>ETPVLEKNNVTLTGGGENVTKELKDKFTSGDFTVVIKYNQSSEKGLQALFGISNSKPGQQNSYVDVFLRDNGELGMEARDTSSNKNNLVSRPASVWGKYKQEAVTNTVAVVADSVKKTYSLYANGTKVVEKKVDNFLNIKDIKGIDYYMLGGVKRAGKTAFGFNGTLENIKFFNSALDEETVKKMTTNAVTGHLIYTANDTTGSNYFRIPVLYTFSNGRVFSSIDARYGGTHDFLNKINIATSYSDDNGKTWTKPKLTLAFDDFAPVPLEWPREVGGRDLQISGGATYIDSVIVEKKNKQVLMFADVMPAGVSFREATRKDSGYKQIDGNYYLKLRKQGDTDYNYTIRENGTVYDDRTNRPTEFSVDKNFGIKQNGNYLTVEQYSVSFENNKKTEYRNGTKVHMNIFYKDALFKVVPTNYIAYISSNDHGESWSAPTLLPPIMGLNRNAPYLGPGRGIIESSTGRILIPSYTGKESAFIYSDDNGASWKVKVVPLPSSWSAEAQFVELSPGVIQAYMRTNNGKIAYLTSKDAGTTWSAPEYLKFVSNPSYGTQLSIINYSQLIDGKKAVILSTPNSTNGRKHGQIWIGLINDDNTIDWRYHHDVDYSNYGYSYSTLTELPNHEIGLMFEKFDSWSRNELHMKNVVPYITFKIEDLKKNL[2x]

S. pneumoniae produces up to three distinct sialidase enzymes: NanA, NanB, and NanC. NanC is an unusual sialidase in that its primary reaction product is 2-deoxy-2,3-didehydro-N-acetylneuraminic acid (Neu5Ac2en, also known as DANA), a nonspecific hydrolytic sialidase inhibitor. NanC adopts the same overall topology as seen in NanA and NanB, with a CBM (residues 85–271), followed by a catalytic domain (residues 272–740). The catalytic domain adopts the canonical glycoside hydrolase family 33 sialidase, six-bladed β-propeller fold shared by viral, bacterial, and mammalian sialidases.

A covalent complex with 3-fluoro-β-N-acetylneuraminic acid is also presented, suggesting a common mechanism with other sialidases up to the final step of product formation. NanC crystals soaked with 2,3-difluoro-N-acetylneuraminic acid (2,3F-Neu5Ac) presented continuous electron density from the ligand C2 position to Tyr-695. 3F-β-Neu5Ac was covalently bound to Tyr-695 in an unstrained 2C5 chair conformation. The covalent bond distance is 1.9 Å. 2,3F-Neu5Ac was also found bound in the CBM binding site. Equivalent complexes have also been observed in the C. perfringens sialidase NanI, the Trypanosoma rangeli sialidase TrSA, and the Trypanosoma cruzi trans-sialidase TcTS. Tyr-695 was confirmed as the nucleophile by soaking a NanC crystal with 2,3F-Neu5Ac, capturing a sialyl-enzyme intermediate with 3F-β-Neu5Ac covalently bound to Tyr-695. The electronegative fluorine atoms at positions C2 and C3 allow trapping of the covalent intermediate by respectively providing a good leaving group and destabilizing the formation of the positive charged transition state required for enzyme desialylation.> SMKETLHIYAASSMTNAVNALVADYSQQHDVKLVTVYGGSSSLARQIEAGAPADLFISANEEWANYLVEKGLVKPNKVVTLAANSLVLIRPTAQPVASFELQDAAAWQTALADSRLAVAQVDAVPAGMYAKQALQHAGVWPELESRLAQTNNVRLALALVERGESPLGIVYKTDALLSDKVTIVTAFSAQSHQPIRYPLAQLNDKAASAEWVAYLRSDAAQQI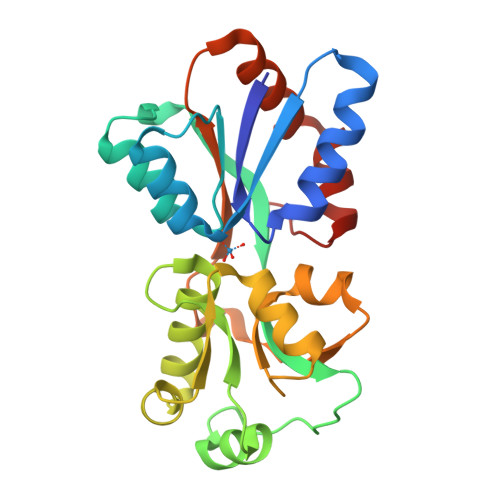LQRFGFESVSE> MALNFTTITENNVIRDLTTQVNNIGEELTKERNIFDITDDLVYNFNKSQKIKLTDDKGLTKSYGNITALRDIKEPGYYYIGARTLATLLDRPDMESLDVVLHVVPLDTSSKVVQH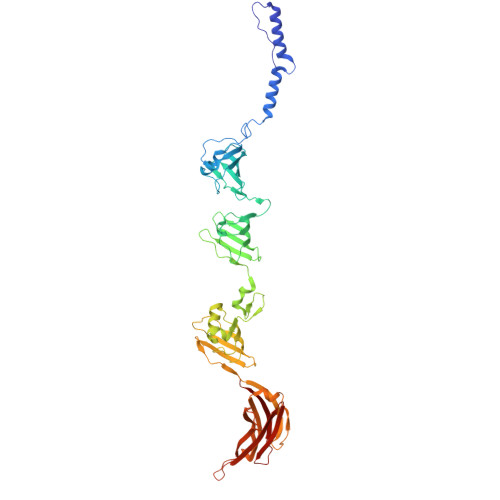LYTLSTNNNQIKMLYRFVSGNSSSEWQFIQGLPSNKNAVISGTNILDIASPGVYFVMGMTGGMPSGVSSGFLDLSVDANDNRLARLTDAETGKEYTSIKKPTGTYTAWKKEFEPKDMEKYLLSSIRDDGSASFPLLVYTSDSKTFQQAIIDHIDRTGQTTFTFYVQGGVSGSPMSNSCRGLFMSDTPNTSSLHGVYNAIGTDGRNVTGSVVGSNWTSPKTSPSHKELWTGAQSFLSTGTTKNLSDDISNYSYVEVYTTHKTTEKTKGNDNTGTICHKFYLDGSGTYVCSGTFVSGDRTDTKPPITEFYRVGVSFKGSTWTLVDSAVQNSKTQYVTRIIGINMP> AVANSIVSSVAPGKEPGSLVCIQAKDGKVIGMGARVHCGPATVLVTAGHVLKKGMIADLYLAKYSVSSKEGKRVLMDPTWKIEYGSLNKEADVISVQVPAAVWSRLGVTAARVRKPTVKVPVLAYGGEASGLLQSSQGFATPDGNMSVAHSCSTRPGWSGTPLYAGSDIVAIHRRWEDIGVKNLATNLSIFHANCASSANGEQGAREIDAEEWISREVTPTDVYIAGRGKYRVAGDEFSHSSYDPLAFSKYKKE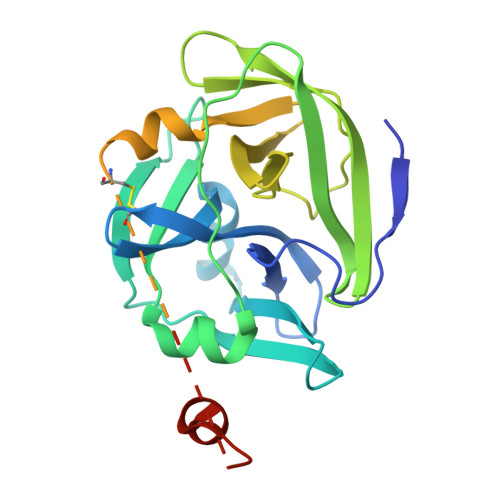RGEMTWADMVEGDLDWDAREE>GSMRHPKIPILKLYNCLLVSIQWELDDQTALTFQEDLLNKIYETGANGVVIDLTSVDMIDSFIAKVLGDVITMSKLMGAKVVLTGIQPAVAVTLIELGIALEEIETALDLEQGLETLKRELGE[5x]

The stressosome transduces environmental stress signals to SigB to upregulate SigB-dependent transcription, which is required for bacterial viability. The stressosome core is composed of RsbS and at least one of the RsbR paralogs. Unlike the RsbR proteins, RsbS only contains an STAS domain. Here, an assembly model of the stressosome is presented based on the crystal structure of the RsbS icosahedron and cryo-EM structures of the RsbRA–RsbS complex determined under diverse symmetry restraints (nonsymmetric C1, dihedral D2 and icosahedral I envelopes).

Cubic crystals belonging to space group I23 were grown under diverse precipitant conditions, such as NaCl, ethanol and polyethylene glycol 8000. Diffraction data were collected to 3.1 Å resolution. Thus, the structure of RsbS was determined by the single-wavelength anomalous dispersion (SAD) method using a crystal of selenomethionine-labeled RsbS. In addition, a β-strand at the N-terminus (β0) interacted with β1 in the manner of an antiparallel β-sheet. In a structural comparison using DALI, RsbS showed high structural similarity to mtSTAS and to Geobacillus stearothermophilus SpoIIAB (gsSpoIIAB), both of which are agonists of antisigma factors. mtSTAS and gsSpoIIAB superimposed onto RsbS with RMSD values of 1.6 and 1.9 Å for 112 Cα positions, respectively [Fig. 1(c)], indicating that RsbS has the conserved fold of the STAS domain. The RsbS crystal contains five monomers in the asymmetric unit. Interface 1 was associated with the formation of the asymmetric unit. A pentameric ring in the asymmetric unit was formed by tandem ‘head-to-tail’ interactions of five RsbS monomers [Fig. 2(b)]. A surface area of 663 Å2 was buried in the binding interface. Interface 2 mediated the interaction between two RsbS pentamers generated by crystallographic symmetry [Fig. 2(b)].>[2x]MSKSDVFHLGLTKNDLQGATLAIVPGDPDRVEKIAALMDKPVKLASHREFTTWRAELDGKPVIVCSTGIGGPSTSIAVEELAQLGIRTFLRIGTTGAIQPHINVGDVLVTTASVRLDGASLHFAPLEFPAVA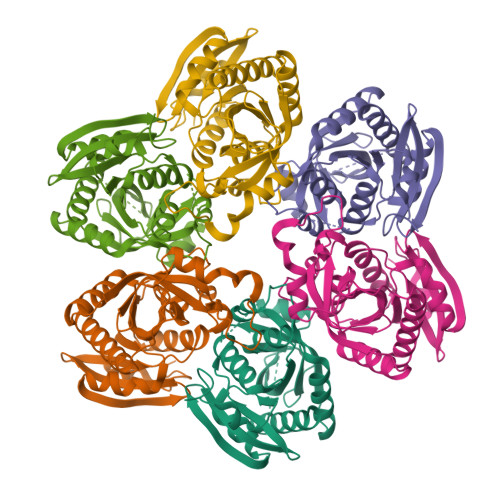DFECTTALVEAAKSIGATTHVGVTASSDTFYPGQERYDTYSGRVVRHFKGSMEEWQAMGVMNYEMESATLLTMCASQGLRAGMVAGVIVNRTQQEIPNAETMKQTESHAVKIVVEAARRLL ARSENATE | As O4 | 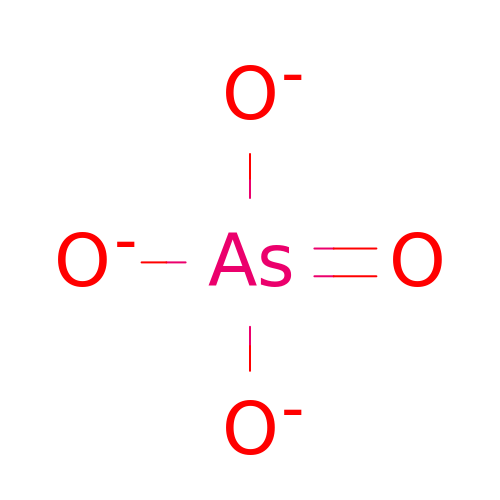DJHGAFSJWGLOIV-UHFFFAOYSA-K>[2x]MDTPNKDDSIIRFSVSLQQNLLDELDNRIIKNGYSSRSELVRDMIREKLV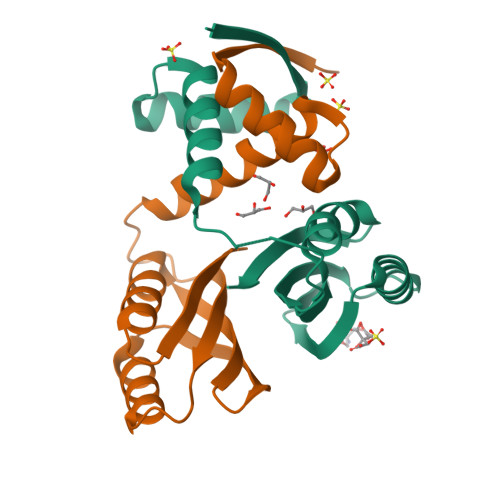EDNWAEDNPNDESKIAVLVVIYDHHQRELNQRMIDIFHASGTHVLCTTHIHMDEHNCLETIILQGNSFEIQRLQLEIGGLRGVKFAKLTKASSFEYNE5,6,7,8-TETRAHYDROBIOPTERIN | C9 H15 N5 O3 | 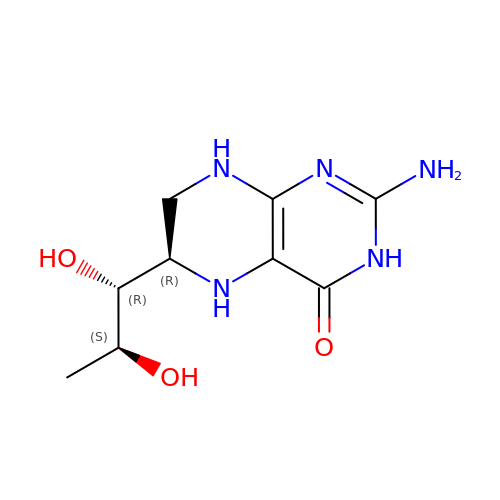FNKQXYHWGSIFBK-RPDRRWSUSA-N> MKRRWKKNFIAVSAANRFKKISSSGALENLYFQGEMEGSTGFDGDATTFFAPDAVFGDRVRRFQEFLDTFTSYRDSVRSIQVYNSNNAANYNDDQDDADERDLLGDDDGDDLEKEKKAASSTSLNILPHRIIISLDDLREFDRSFWSGILVEPAYFIPPAEKALTDLADSMDDVPHPNASAVSSRHPWKLSFKGSFGAHALSPRTLTAQHLNKLVSVEGIVTKTSLVRPKLIRSVHYAAKTGRFHYRDYTDATTTLTTRIPTPAIYPTEDTEGNKLTTEYGYSTFIDHQRITVQEMPEMAPAGQLPRSIDVILDDDLVDKTKPGDRVNVVGVFKSLGAGGMNQSNSNTLIGFKTLILGNTVYPLHARSTGVAARQMLTDFDIRNINKLSKKKDIFDILSQSLAPSIYGHDHIKKAILLMLMGGVEKNLENGSHLRGDINILMVGDPSTAKSQLLRFVLNTASLAIATTGRGSSGVGLTAAVTTDRET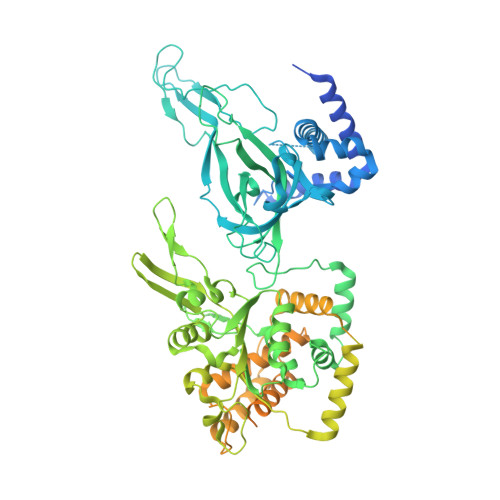GERRLEAGAMVLADRGVVCIDEFDKMTDVDRVAIHEVMEQQTVTIAKAGIHTTLNARCSVIAAANPVFGQYDVNRDPHQNIALPDSLLSRFDLLFVVTDDINEIRDRSISEHVLRTHRYLPPGYLEGEPVRERLNLSLAVGEDADINPEEHSNSGAGVENEGEDDEDHVFEKFNPLLQAGAKLAKNKGNYNGTEIPKLVTIPFLRKYVQYAKERVIPQLTQEAINVIVKNYTDLRNDDNTKKSPITARTLETLIRLATAHAKVRLSKTVNKVDAKVAANLLRFALLGEDIGNDIDEEESEYEEALSKRSPQKSPKKRQRVRQPASNSGSPIKSTPRRSTASSVNATPSSARRILRFQDDEQNAGEDDNDIMSPLPADEEAELQRRLQLGLRVSPRRREHLHAPEEGSSGPLTEVGTPRLPNVSSAGQDDEQQQSVISFDNVEPGTISTGRLSLISGIIARLMQTEIFEEESYPVASLFERINEELPEEEKFSAQEYLAGLKIMSDRNNLMVADDKVWRV>[2x]MKHHHHHHQMFKKVLVANRGEIACRVIRACKELGIQTVAIYNEIESTARHVKMADEAYMIGVNPLDTYLNAERIVDLALEVGAEAIHPGYGFLAENEHFARLCEEKGITFIGPHWKVIELMGDKARSKEVMKRAGVPTVPGSDGILKDVEEAKRIAKEIGYPVLLKASAGGGGRGIRICRNEEELVRNYENAYNEAVKAFGRGDLLLEKYIENPKHIEFQVLGDKYGNVIHLGERDCSIQRRNQKLVEI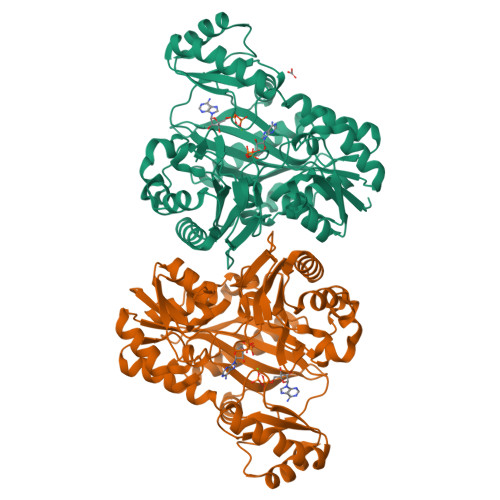APSLLLTPEQREYYGSLVVKAAKEIGYYSAGTMEFIADEKGNLYFIEMNTRIQVEHPVTEMITGVDIVKWQIRIAAGERLRYSQEDIRFNGYSIECRINAEDPKKGFAPSIGTIERYYVPGGFGIRVEHASSKGYEITPYYDSLIAKLIVWAPLWEVAVDRMRSALETYEISGVKTTIPLLINIMKDKDFRDGKFTTRYLEEHPHVFDYAEHRDKEDFVAFISAVIASYHGL>[2x]SVKDEAK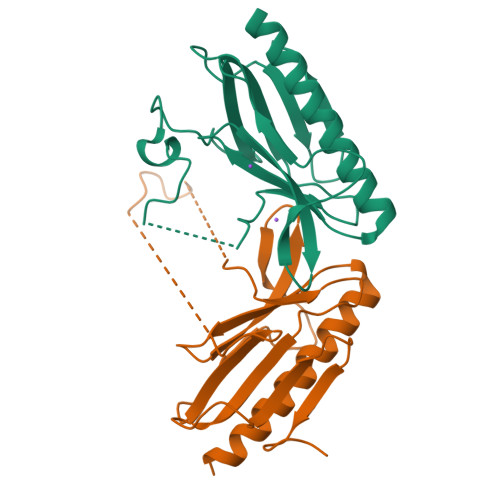ISAQSFYQRLLLLNEEAILSGQDFGVRIDVDTRRLTFLQLTADKGWQKWQNDKMTNQTTLKEGLQLDFELGGGAWQKDDRLFNPGSLFDEEMFADEKKEQKQEPAPQLFVLSSGEVTPFTLSIFPKGQEPDEQWRVTAQENGTLRLLAPGESDEELEHHHHHH> MRGSHHHHHHGSGSMGMTLETAFMLPVQDAQHSFRRLLKAMSEPGVIVALHQLKRGWQPLNIATTSVLLTLADNDTPVWLSTPLNNDIVNQSLRFHTNAPLVSQPEQATFAVTDEAISSEQLNALSTGTAVAPEAGATLILQ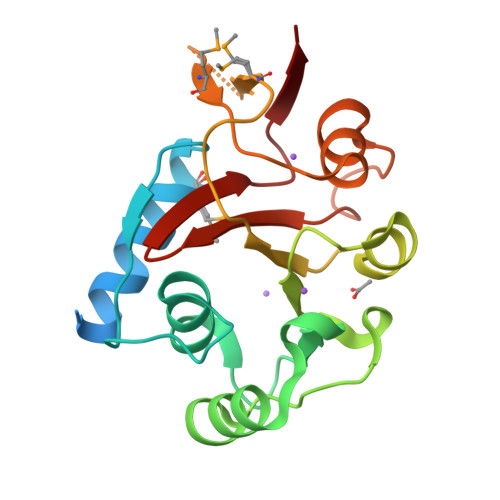VASLSGGRMLRLTGAGIAEERMIAPQLPECILHELTERPHPFPLGIDLILTCGERLLAIPRTTHVEVC> TPAFNKPKVELHVHLDGAIKPETILYFGKKRGIALPADTVEELRNIIGMDKPLSLPGFLAKFDYYMPVIAGCREAIKRIAYEFVEMKAKEGVVYVEVRYSPHLLANSKVDPMPWNQTEGDVTPDDVVDLVNQGLQEGEQAFGIKVRSILCCMRHQPSWSLEVLELCKKYNQKTVVAMDLAGDETIEGSSLFPGHVEAYEGAVKNGIHRTVHAGEVGS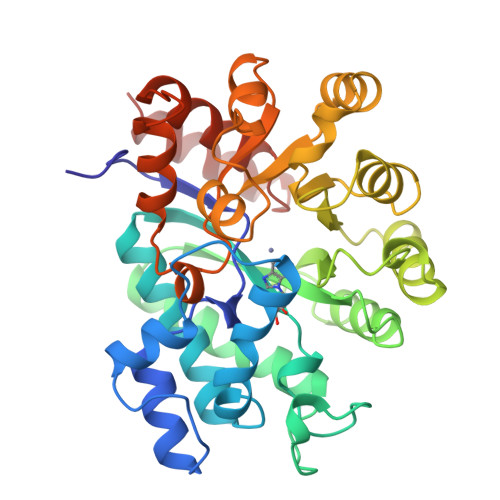PEVVREAVDILKTERVGHGYHTIEDEALYNRLLKENMHFEVCPWSSYLTGAWDPKTTHAVVRFKNDKANYSLNTEDPLIFKSTLDTDYQMTKKDMGFTEEEFKRLNINAAKSSFLPEEEKKELLERLYREYQ> MAFAGAAAPLGVKGRSVFAGMRSFIGQRLGRLYDSFYYSQSSTKYVMVFLFPAGIFYTRFRADTKLGYHVFINEEKLYP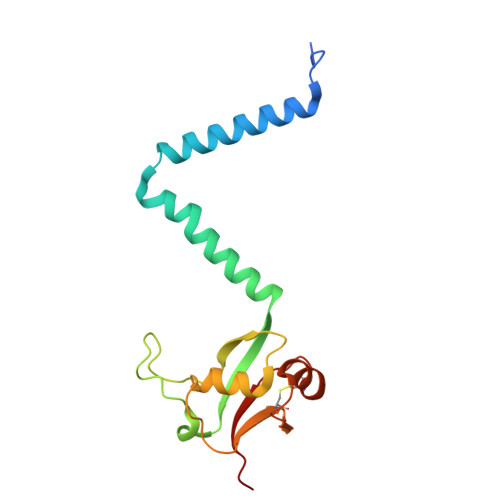DYSQNYFDTKWTNGRKVYLDDETTVEQLKAQIYGGKAAPENVKVACRGRVFEDADNVAMAVRAFCKRDPRLLLFQDNL>[4x]SHAGANDLCQECEDIVHLLTKMTKEDAFQEAIRKFLEQECDI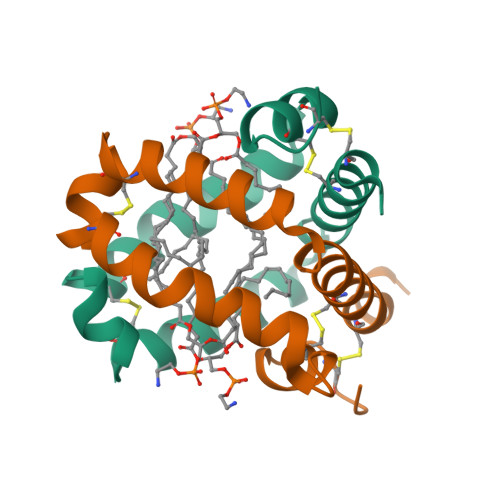LPLELLVPECRQVLDVYLPLVIDYFQSQINPKAICNHVGLCPRGQ> QYNNQN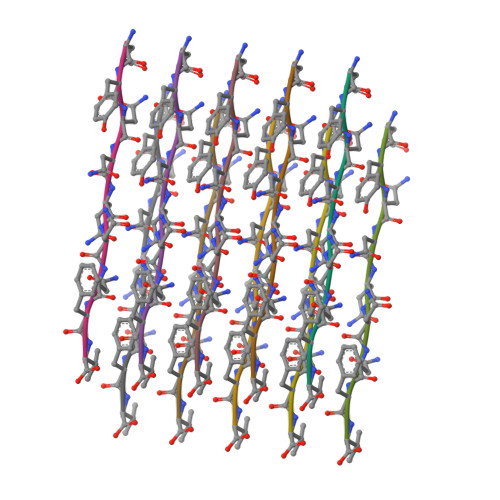NFV> CPERELQRREEEANVVLTGTVEEIMNVDPVHHTYSCKVRVWRYLKGKDIVTHEILLDGGNKVVIGGFGDPLICDNQVSTGDTRIFFVNPAPQYMWPAHRNELMLNSSLMRITLR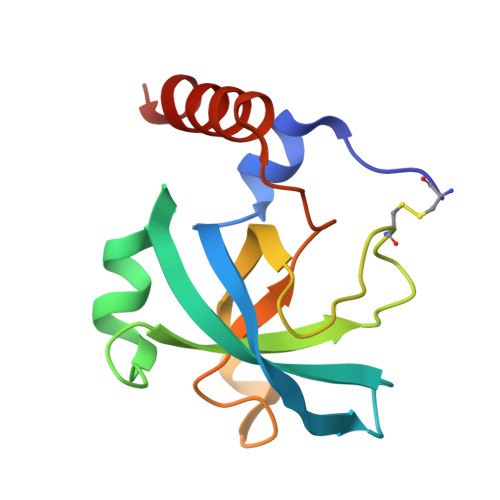NLEEVEHCVEEHRK>[3x]VMLQPYKHEPFTDFTVEANRKAFEEALGLVEKELGKEYPLIINGERVTTEDKIQSWNPARKDQLVGSVSKANQDLAEKAIQSADEAFQTWRNVNPEERANILVKAAAIIRRRKHEFSAWLVHEAGKPWKEADADTAEAIDFLEYYARQMIELNRGKEILSRPGEQNRYFYTPMGVTVTISPWNFALAIMVGTAVAPIV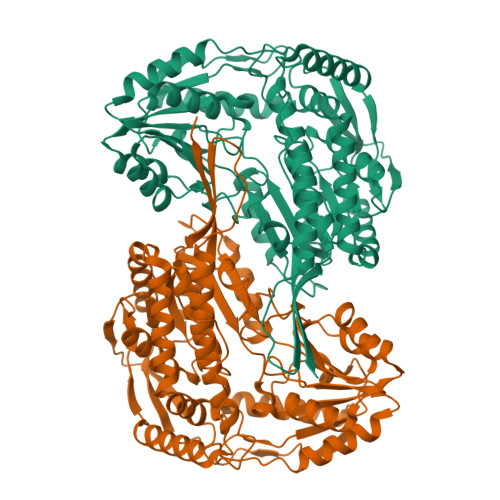TGNTVVLKPASTTPVVAAKFVEVLEDAGLPKGVINYVPGSGAEVGDYLVDHPKTSLITFTGSKDVGVRLYERAAVVRPGQNHLKRVIVEMGGKDTVVVDRDADLDLAAESILVSAFGFSGQKCSAGSRAVIHKDVYDEVLEKTVALAKNLTVGDPTNRDNYMGPVIDEKAFEKIMSYIEIGKKEGRLMTGGEGDSSTGFFIQPTIIADLDPEAVIMQEEIFGPVVAFSKANDFDHALEIANNTEYGLTGAVITRNRAHIEQAKREFHVGNLYFNRNCTGAIVGYHPFGGFKMSGTDSKAGGPDYLALHMQAKTVSEMYAENLYFQSHHHHHHWSHPQFEK> MQGSRKPNIIFIMADDLGWGELGSYGNTFNETPNLDRLSAQGMRFTQAYAAAPVASPTRASIMTGQYPARVGITDFLPEDEKTDRWLDPTKYVTLNEALSASGYHTGIVGKWHLDTDFKLNKGGPKAHGFNEVIGTESEYIADGDYFFPYSKIASFDKGTANEYLTDRQCAEANAFITRNREKPFFLYLSLYSVHTRLEAPVQLVEKYKQKFDQKYGTGKAEQFFGANNVRHESAQRDNPWLAAMLESIDTGVGGIMKTLRETGLAENTIIVFFSDNGGAGKAGNNAHLRAGKTWLYEGGIREPLIVSWPGKIKGNTVNDNPVTSLDFYPTFLAAAGGKPTGGRLDGHNLMPLLRGGRASGRPLFWHYPSETGKWVNRMSSAVREGNYKLLEFYNNPRLELYDLQNDPSESHNLATDRPAETARLKKLLEDWKKEVNAEAPHLARKEKKKPGSHHHHHH

We expressed and characterized a putative sulfatase (PyuS) from the bacterium Pedobacter yulinensis. PyuS contains the (C/S)XPXR sulfatase motif, where the Cys or Ser is post-translationally converted into a formylglycine residue (FGly). The enzyme has sulfatase activity on aromatic sulfated substrates as well as phosphatase activity on some aromatic phosphates; however, PyuS did not have detectable activity on 17α-estradiol sulfate, cortisol 21-sulfate, or boldenone sulfate. The PyuS protein chain has an α/β sandwich fold comprised of 15 α-helices and 13 β-strands that form two anti-parallel β-sheets.

Furthermore, we were able to obtain three high-resolution crystal structures of PyuS. The protein crystallized in the P3221 space group with one protein chain per asymmetric unit for all structures. The crystal structure of PyuS shows that the active-site cysteine is converted to formyl-glycine. However, with no sulfate substrate bound in the active site, the expected 2-amino-3-oxopropanoic has been oxidized to a hemi-acetal functional group. In addition, the analysis of the electron density maps, B-factors, and geometry of the metal binding site allowed us to identify Ca2+ as being present in the active site. Our structural studies indicate that negatively charged entities such as malonate, bromine, and citrate are favored ligands for binding to the PyuS active site, and these ligands are in the vicinity of active site residues His195 and Lys293. This is not surprising as they mimic sulfate or the phosphate moieties of sulfatase or phosphatase substrates, respectively, and the active site of PyuS has an overall positive charge. The PDBePISA analysis of PyuS crystal structures revealed that PyuS forms homodimers. Dimers are also seen in the crystal structures, and PDBePISA shows that the interface area between monomers in the crystal structure exceeds the threshold to distinguish between real dimers and experimental artifacts. In all of the PyuS crystal structures, there is at least one type of ion (sodium, bromine, or chloride) present in the putative dimer interface, and these ions may help facilitate dimer formation.>SNAMEPVSSWGNTSLVSVDPEIHDLIEKEKRRQCRGIELIASENFTSFAVIEALGSALTNKYSEGIPGNRYYGGNEFIDEIENLCRSRALEAFHCDPAAWGVNVQPYSGSPANFAAYTALLQPHDRIMGLDLPSGGHLTHGYYTSGGKKISATSIYFESLPYKVNFTTGYIDYDKLEEKALDFRPKLLICGGSAYPRDWDYARFRAIADKVGALLLCDMAHISGLVAAQEAANPFEYCDVVTTTTHKSLRGPRAGMIFYRKGPKPPKKGQPEGAVYDFEDKINFAVFPALQGGPHNHQIGALAVALKQANTPGFKVYAKQVKANAVALGNYLMSKGYQIVTNGTENHLVLWDLRPLGLTGNKVEKLCDLCSITLNKNAVFGDSSALAPGGVRIGAPAMTSRGLVEKDFEQIGEFLSRAVTLTLDIQKTYGKLLKDFN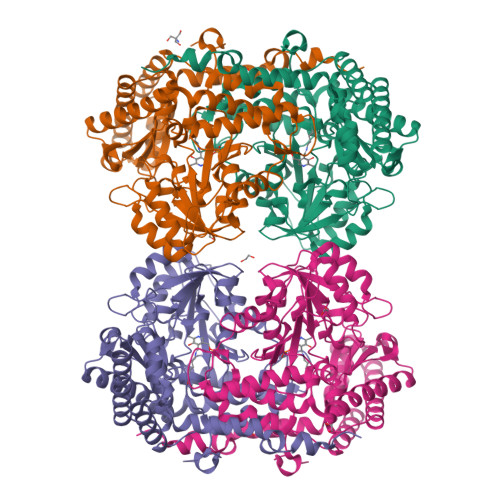KGLVNNKDLDQLKADVEKFSASYEMPGFLMSEMKYKD[4x]>[4x]HSTEEGLFSQKSFLVLGFSNENESNIANIIKENAGKIMSLLSRTVADYAVVPLLGCEVEATVGEVVTNTWLVTCIDYQTLFDPKSNPLFTPVPVMTGMTPLEDCVISFSQCAGAEKESLTFLANLLGASVQEYFVRKSNAKKGMFASTHLILKERGGSKYEAAKKWNLPAVTIAWLLETARTGKRADESHFLIENS;>SSDLVAPSPDAFRST[2x]

53BP1 and TOPBP1 are multi-domain scaffold proteins that individually contribute to the genome stability functions of mammalian cells. Amongst other roles, TOPBP1 is involved in replication initiation through its interaction with TICCR/Treslin; the DNA damage checkpoint through interactions with 9-1-1, RHNO1/RHINO and ATR; and sister chromatid de-catenation and suppression of sister chromatid exchange via interactions with TOP2A and BLM. 53BP1 is recruited to sites of DNA damage through interaction with post-translationally modified histones and is strongly implicated in the process of choice between the non-homologous end joining and homologous recombination pathways of double-strand break (DSB) repair, as well as the localisation of activated ATM that is required for DSB repair in heterochromatin. Using a structurally-derived consensus pattern for phospho-ligand binding to the N-terminal regions of TOPBP1 and Rad4, we have now identified conserved phosphorylation sites in human 53BP1, and have biochemically and structurally characterised their interaction with BRCT domains of TOPBP1.

However, the 53BP1-pSer366 peptide did show a clear interaction with TOPBP1-BRCT4,5, albeit with a more modest affinity (Kd = 20.6 ± 1.9 μM). Treatment of the phosphopeptide with λ-phosphatase or mutation of Lys704, which is implicated in phosphate recognition in TOPBP1-BRCT4,5 eliminated binding, confirming the phospho-specificity of the interaction. We were also able to obtain co-crystals of the 53BP1-pSer366 peptide bound to TOPBP1-BRCT4,5. The 53BP1-pSer366 peptide binds to BRCT5 in a similar position and orientation as previously observed for phospho-peptide binding to TOPBP1-BRCT1 and BRCT2 (see above) and Rad4-BRCT1 and BRCT2. The phosphoserine side chain engages with the topologically conserved TOPBP1-Ser654 and with the side chain of TOPBP1-Lys704. The −3 residue in the bound peptide, 53BP1-Val363, binds into a hydrophobic pocket lined by the side chains of TOPBP1 residues Phe673, Ser703, Lys704, Ala707 and Trp711. Additional specificity is provided by the hydrophobic packing of the side chains of 53BP1 residues Ala364 and Pro365 around the protruding side chain of TOPBP1-Tyr678, and the packing of 53BP1-Leu362 into a hydrophobic pocket formed by the side chains of TOPBP1-Tyr678, Val680 and Met689. The identified binding site in BLM - 300-FVPPpSPE-306 shows strong similarity to the 53BP1-motif we have identified - 362-LVAPpSPD-368, and binds to BRCT5 in a very similar manner, but quite differently from the proposed binding mode of the MDC1 SDT motif, which we have recently shown plays no role in mediating MDC1 interaction with TOPBP1.>MASMTGSAKLISVTKPVVEGVNTAEELIAYAARVSNPENQINNKTASGLLKYCIRHKHWSIFETAFMTLELKTSRGIAAQVLRHRSFHFQEFSQRYASVMETPPPHQARFQDHKNRQNSLDTVPEDDQTWWATEQEKLYAQSMELYNKALEKGIAKECARFILPLSTPTTIYMSGTIRDWIHYIELRTSNGTQREHIDLANACKEIFIKEFPSIAKALDWVHHHHHH[16x]

The last step of dTMP synthesis is the methylation of 2′-deoxyuridine-5′-monophosphate (dUMP) to dTMP. This N5,N10-methylene-5,6,7,8-tetrahydrofolate (CH2H4folate)-dependent reaction is catalysed by two distinct families of thymidylate synthases, ThyA (EC 2.1.1.45) and ThyX (EC 2.1.1.148; flavin-dependent thymidylate synthase (FDTS)), without detectable sequence or structural similarity. Whereas human and bacterial ThyA proteins use tetrahydrofolate (H4folate) to reduce the methylene moiety after its transfer to the uracil ring, ThyX proteins use a non-covalently bound flavin adenine dinucleotide (FAD) cofactor to facilitate hydride transfer from NAD(P)H. Recent studies have demonstrated accumulation of a 5-hydroxymethyl-dUMP (5hmdUMP) as an acid-trapped intermediate during ThyX catalysis. ThyX has a complex fold with a central a/b domain flanked by two helical domains. It forms a tetramer with a 222 symmetry.

In order to obtain further insight into the mechanism of ThyX inhibition, we solved the crystal structure of C8-C1 bound to PBCV-1 ThyX at a resolution of 2.6 Å. The space group was P1 with four ThyX homotetramers per asymmetric unit. C8-C1 binds within the catalytic pocket between two ThyX monomers (hereafter called monomer A and B). The C8-C1 binding site is conserved and partially overlaps with the dUMP binding pocket observed in T. maritima and M. tuberculosis ThyX. The 1,4-NQ moiety binds in the same cavity as the uracil ring from dUMP and is sandwiched between the FAD isoalloxazine ring on one side and side chains from Gln-75 (monomer A) and Gln-89 (monomer B) on the other side. The binding of the 1,4-NQ moiety is further stabilized by four hydrogen bonds: the carbonyl group at position 4 interacts with the hydroxyl group from Ser-88 and the main chain N from Gln-89 in monomer B. On the opposite side of the ring, the Arg-182 side chain from monomer A forms hydrogen bonds with the 1,4-NQ carbonyl and hydroxyl groups at positions 1 and 2, respectively. The aliphatic parts of the Gln-75, Glu-152 and Arg-90 side chains form the wall of a hydrophobic pocket that accommodates the 4-methoxybenzyl group of C8-C1. This pocket is distinct from the one accommodating the dUMP phosphoribose moiety; hence, the binding mode of the inhibitor is distinct from dUMP binding. Comparison with the structure of the FAD-bound form of PBCV-1 ThyX shows that upon inhibitor binding, a long loop located in the vicinity of the substrate binding site (residues 89–104) becomes ordered and participates in C8-C1 binding. When the IC50 at a fixed enzyme concentration was plotted as a function of the dUMP concentration (indicated as [S]/km), a linear correlation with a positive slope (r2 ≈ 0.97) was observed, indicating that the molecule C8-C1 acts as a tight-binding competitive inhibitor with respect to dUMP.> AVKYYTLEEIQKHNNS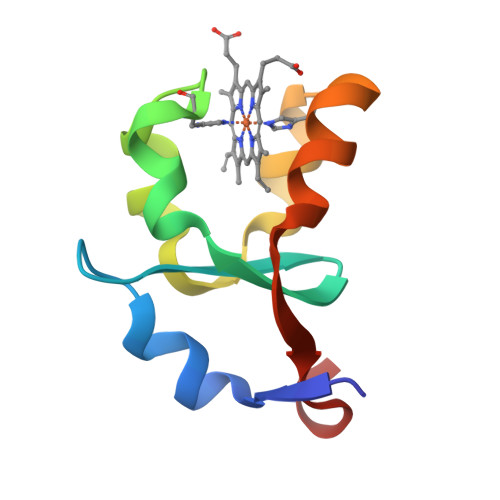KSTWLILHYKVYDLTKFLEEHPGGEAVLRAQAGGDATANFEAVGHSTDARELSKTFIIGELHPDDR>ADTRIGVTIYKYDDNFMSVVRKAIEKDGKSAPDVQLLMNDSQNDQSKQNDQIDVLLAKGVKALAINLVDPAAAGTVIEKARGQNVPVVFFNKEPSRKALDSYDKAYYVGTDSKESGVIQGDLIAKHWQANQGWDLNKDGKIQYVLLKGEPGHPDAEARTTYVVKELNDKGIQTEQLALDTAMWDTAQAKDKMDAWLSGPNANKIEVVIANNDAMAMGAVEALKAHNKSSIP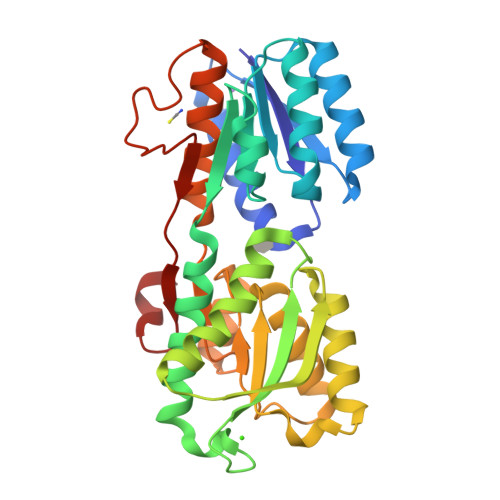VFGVDALPEALALVKSGAMAGTVLNDANNQAKATFDLAKNLAEGKGAADGTSWKIENKIVRVPYVGVDKDNLSEFTQK[2x]>[7x]MAIAQLATEYVFSDFLLKEPTEPKFKGLRLELAVDKMVTCIAVGLPLLLISLAFAQEISIGTQISCFSPSSFSWRQAAFVDSYCWAAVQQKNSLQSESGNLPLWLHKFFPYILLLFAILLYLPPLFWRFAAAPHICSDLKFIMEELDKVYNRAIKAAKSARDLDMRDGACSVPGVTENLGQSLWEVSESHFKY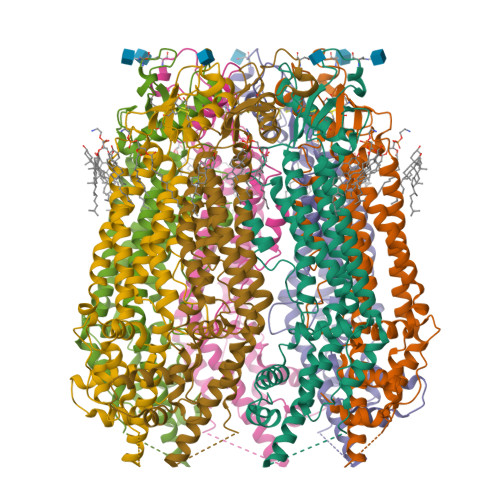PIVEQYLKTKKNSNNLIIKYISCRLLTLIIILLACIYLGYYFSLSSLSDEFVCSIKSGILRNDSTVPDQFQCKLIAVGIFQLLSVINLVVYVLLAPVVVYTLFVPFRQKTDVLKVYEILPTFDVLHFKSEGYNDLSLYNLFLEENISEVKSYKCLKVLENIKSSGQGIDPMLLLTNLGMIKMDVVDGKTPMSAEMREEQGNQTAELQGMNIDSETKANNGEKNARQRLLDSSC> NLYQFKNMIQCTVPSRSWCDFADYGCYCGKGGSGTPVDDLDRCCQVHDNCYNEAEKISGCWPYFKTYSYECSQGTLTCKGGNNACAAAVCDCDRLAAICFAGAPYTDANYNIDLK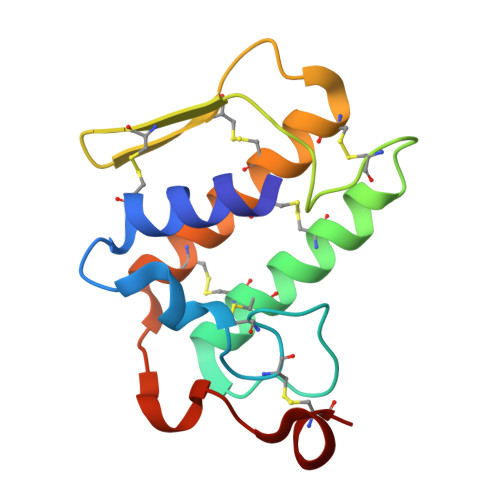ARCQ> MEQTLAILKNDNSTLVAEMQNQLVHDFSPNGTALPELDIKAFVQKLGQRLCHRPYVYSAFMDVVKALHNEIVDFPGFIERISVILRDYPDLLEYLNIFLPSSYKYLLSNSGANFTLQFTTPSGPVSTPSTYVATYNDLPCTYHRAIGFVSRVRRALLSNPEQFFKLQDSLRKFKNSECSLSELQTIVTSLLAEHPSLAHEFHNFLPSSIFFGSKPPLGSFPLRGIQSSQFTLSNISDLLSQSRPDNLSPFSHLSNESSDFFKNVKNVLTDVETYHEFLKLLNLYVQGIIDRNILVSRGFGFLKSNSGLWRSFLSLTSLSPEEFLSVYNSACSDFPECGPSYRLLPVEERNISCSGRDDFAWGILNDDWVSHPTWASEESGFIVQRKTPYEEAMTKLEEERYEFDRHIEATSWTIKSLKKIQNRINELPEEERETYTLEEGLGLPSKSIYKKTIKLVYTSEHAEEMFKALERMPCLTLPLVISRLEEKNEEWKSVKRSLQPGWRSIEFKNYDKSLDSQCVYFKARDKKNVSSKFLLAEADILRSQAKLHFPLRSRSAFEFSFVYDNEIVLFDTCYMVCTYIVCNSPSGLKKVEHFFKNILPLHFGLEKDKFSIFLDQVFRGPDYDVNAPNIVGNKPVRRKRSNSITQLTEFVKQPKINGQRESRSAAAARKKEESGNKSQSNSQNSLSDESGNVTPVSKKQLSQPAAAIKASLKYPSHPDSLLEHQDHAGDTENEMHDDVDKEQFGYSSMYVFFRLFNLLYERLYELQRLEDQVSIIQQRIIPNPVSQKQKIWRDRWNDLSDVPDEKTHYENTYVMILRLIYGIVDQSAFEDYLRFYYGNKAYKIYTIDKLVWSAAKQVHHIVSDGKYKFVTSLVEQNSSASPKKNYDDFLYRLEIEKLLNPDEILFRFCWINKFKSFGIKIMKRANLIVDQSLDTQRRVWKKYVQNYRIQKLTEEISYKNYRCPFLCRNIEKERTVEQLVSRLQTKLLRSAELVSGLQAKLCLDSFKLLYLPRTEDSYIDASYLRLRDTDFLDCQNKRKQRWRNRWESLLKSVRGTSDNTAEVNFDADINALFIP;> MGFGKKKVSYFYDEDVGNYHYGPQHPMKPHRVRMVHNLVVNYNLYEKLNVITPVRATRNDMTRCHTDEYIEFLWRVTPDTMEKFQPHQLKFNVGDDCPVFDGLYEFCSISAGGSIGAAQELNSGNAEIAINWAGGLHHAKKREASGFCYVNDIALAALELLKYHQRVLYIDIDVHHGDGVEEFFYTTDRVMTCSFHKFGEYFPGTGHIKDTGIGTGKNYAVNVPLRDGIDDESYESVFKPVISHIMQWFRPEAVILQCGTDSLAGDRLGCFNLSMKGHSMCVDFVKSFNLPMICVGGGGYTVRNVARVWTYETGLLAGEELDENLPYNDYLQYYGPDYKLNVLSNNMENHNTRQYLDSITSEIIENLRNLSFAPSVQMHKTPGDFTFENAEKQNIAKEEIMDERV;> MAVSAVPHPSKQAQASEEGINQEKCINEEYKIWKKNSPFLYDLIITRALEWPCMSLQWYPEQQIFAEHGYTEQKMFLGVRADVGKYLLAVASIQLPYLNQTVPPTTMEGASAGDESSLRVNISNLYSHPESVCSAKLMPQDDSCVATVGNYHNDVLVFDKESFESYSSASESPLKPKYRLTKHTQPCTSVCWNFLSKGTLVSGSQDATLSCWDLNAYNESDSASVLKVHISSHEKQVSDVRFHYKHQDLLASVSYDQYLHVHDIRRPDASTKPARSVHAHSGPIHSVAFNPHNDFILATCSTDKTIALWDLRNLNQRLHTLEGHEDIVTKISFSPHEEPILASTSADRRTLVWDLSRIGEDQPAEEAQDGPPELLFMHGGHTSCTIDMDWCPNYNWTMATAAEDNILQIWTPSRSIWGNEQLEEDATAYLS;>MAVSYKVNERVLCFHGPLLYEAKIVDTEMKGDVTTYLIHYKGWKNSWDEWVEQDRILQWTEENLKTQKELKNAAISTRQKPTSKKSASSTSKHDSTGVKTSGKRSRESSTVTVDGDSHELPSRIKTQKSESPIPQQVKRDGTTDAKNEETTKPENNEKDDFEEEPPLPKHKISVPDVLKLWLVDDWENITKNQQLIAIPRNPTVRAAIAAFRESKISHLNNEIDVDVFEQAMAGLVIYFNKCLGNMLLYRFERQQYLEIRQQYPDTEMCDLYGVEHLIRLFVSLPELIDRTNMDSQSIECLLNYIEEFLKYLVLHKDEYFIKEYQNAPPNYRSLVGV[2x];> MASSINNSSQPTVPSISNNSHGDSFVNEGPPSNFKNNSLTSSTHSSTDHVNVLPISQDKEMDISSPVKKQKASYSNKSPNKAPIQKSRGSSLKSHLETESQQTPVKRRRRKATIRNVDYCSACGGRGLFICCEGCPCSFHLSCLEPPLTPENIPEGSWFCVTCSIKSHHPPKHPLSIWSQLYDWIDSQNPSQYRLPDDLVHYFHGISRGDTGAYKETEGEMDTDEFSALPTGSSITNLAYCGYCSKPSMGACWVYGCQLCDTFYHKNCKEHAKKCSHDSIGKKGMRVPKNAVVIRTPLVLDTTSNTLNPKVMISGWQFLMGEFPSDELLYFPRLPVSCLYKVSEDGLIKDFLYAIGIEAKKFNNERKKRELEVIPPDVKSALLPARTHPNLPIALRTLFNKART;> MDAKPWNHTSEAFQASILEDLKIIQKAGAERNAKSSHGSINSRSASPNKATSRRNRAQNGNSNGRASVDNSDDGSKDDLDYSPSVKRKHVNGEGAEKGDHDTSNNGPSITKLRRKVRRTYDTKDGFVAWNTLDDDFRPIVPDQERSRKINPQKGNNNNLLKENKSLKTTAKDLSDISSSSMKKANNSSKPLFSGKLTFKANIPVPTSEVVTENNVTRNVTVYSNQKHLGNESENFNDMEGRAEDISSNELLPTPEEYPYRYNNDYCSACHGPGNFLCCETCPNSFHFTCIDPPIEEKNLPDDAWYCNECKHHSLYNELDEQEELESNVKEEGTMVDVWMQLCTYIDSHNPIQFHLPHSISSFFRGVGSGVMGEYIETDVLKHLKSSRRSNGEERDPLLLKSKSGTPILCFRCHKSALVSQSILACDYCNSYWHPDCLNPPLATLPSNLRKWKCPNHSDHVTPRYRLPEKAKVIRVGLPRGFKNKGNIVIDENEDEPSVQTIQLQGKIRVVPSKPFKLNFLEQIRDNVINLRKMVEQDEQLCIETFSKFDFYATRDCELPLRILCDVANDNLENDDYVLALRDLLRISKWDPNQPVPAPFDLANLLSY

The switch-independent 3 (SIN3)/histone deacetylase (HDAC) complexes are chromatin modifiers that catalyze local histone deacetylation and regulate global gene expression. The highly conserved, multidomain-containing protein Sin3 is thought to provide a platform for the assembly of HDACs and non-catalytic subunits, forming two major types of the SIN3/HDAC complexes (SIN3L and SIN3S). The histone deacetylase Clr6 belongs to the zinc-dependent class I HDAC family, which serves as the catalytic subunits of multiple transcriptional regulatory complexes, such as SIN3, NuRD, CoREST, SMRT/NCoR and MiDAC. In each lobe, the Sin3 isoform (Pst1, Pst2, or Pst3) wraps up Clr6 through its HID and binds to the Prw1 through its HCR.

We sought to purify the endogenous SIN3/HDAC complexes from S. pombe by employing a C-terminal Flag-tag on the Sin3 homolog Pst1, Pst2, or Pst3. Cryo-EM analysis finally yielded a reconstruction of SIN3L at an average resolution of 3.2 Å from the Pst3-Flag yeast strain and a map of the SIN3S at 2.9 Å resolution from the Pst2-Flag yeast strain. In the structure of SIN3S, Pst2 organizes Clr6, Prw1, Cph1, Cph2, and two copies of Eaf3 (Eaf3 and Eaf3’), assembling into a delicate ‘Small’ scaffold. Unlike the SIN3L complex, the SIN3S complex reveals a compact organization with four modules: the Pst2 Lobe (Pst2_HID/HCR, Clr6, and Prw1), two histone binding modules (the HB1 module, consisting of Cph1_NTD and Eaf3, and the HB2 module, consisting of Cph2_NTD and Eaf3’), and a scaffold (Pst2_PAH1–3, Cph1_CTD, and Cph2_CTD). Similar to the Pst1 in the SIN3L, the HID of Pst2 binds to the Clr6 and the HCR interacts with Prw1, forming the Pst2 Lobe. The PAH1/2/3 of Pst2 respectively stabilizes Cph2_α4, Cph2_α5, or Cph1_α4 in the rear side of the deacetylase activity center, constructing the scaffold to bridge the Pst2 Lobe and the HB1/2 modules (Fig. 3b, Side View). In addition, the Cph1_β3 forms a β-sheet with the Cph2_β5–6, and the Cph1_α5 interacts with the Cph2_α6–7, forming two junctions to further stabilize the whole complex. The Cph1_NTD (consisting of PHD, SID, and BR) and the Cph2_NTD (consisting of PHD1, SID, and PHD2) respectively recruit the MRG domains of Eaf3 and Eaf3’ through their SIDs (α2–3), forming two separate modules. The highly conserved residues Asp118 of Cph1 and Asp264 of Cph2 may recognize and bind to the residue Lys4 of the H3 histone. While in SIN3S, Junction 2 of Cph1 and Cph2 serves as the third anchor (the other two refer to the HID1 and HID2 of Pst2) to stabilize the Clr6. The HB1 and HB2 of the SIN3S complex may offer two binding sites for the adjacent nucleosomes with H3K36me3 markers.> AFDAFLKIDGIPGESSDDKHKDWIEIQSFAHKLEQPAQATASSAGGATAERVNHAAYEITHFLDKASPKIYEACCKGQHIKEITIELCRAGGDKVKYMEIKMEQVLIAKVEPHGSANDNGFPSEKVSFTYGKIKWTYTQQKRADGAGGGNVSSG;>[5x]AFDAFLKIDGIPGESSDDKHKDWIEIQSFAHKLEQPAQAT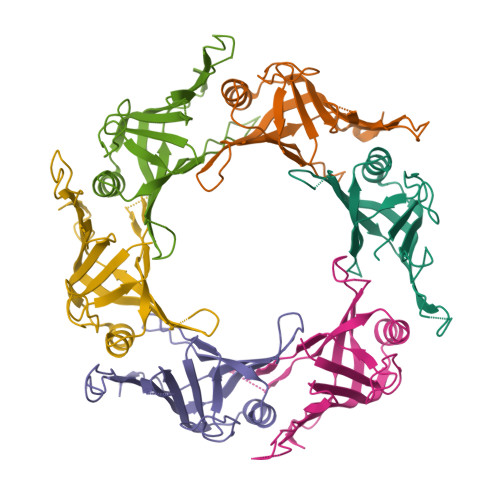ASSAGGATAERVNHAAYEITHFLDKASPKIYEACCKGQHIKEITIELCRAGGDKVKYMEIKMEQVLIAKVEPHGSANDNGFPSEKVSFTYGKIKWTYTQQKRADGAGGGNVSSGWDLTANKAI> LLKALKKLAK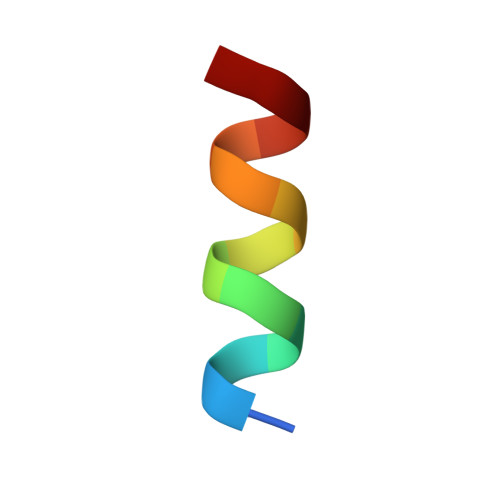KYK> MAALGHTLP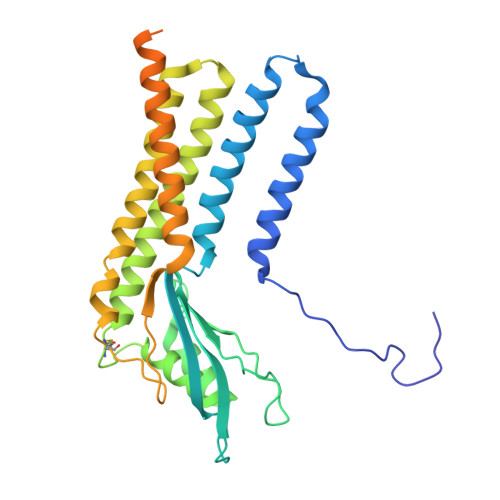FYTGTKPTFPMDTTLAVIITIFLTALVTFIIILPGIRGKTRLFWLLRVVTSLFIGAVILAVNFSSEWSVGHVNANTTYKAFSPKWVSVDVGLQIGLGGVNITLTGTPVQQLNETINYNEAFAWRLGRSYAEEYAKALEKGLPDPVLYLAEKFTPRSPCGLYNQYRLAGHYASAMLWVAFLCWLLANVMLSMPVLVYGGHMLLATGLFQLLALFFFSMTTSLISPCPLRLGTAVLHTHHGPAFWITLATGLLCILLGLVMAVAHRMQPHRLKAFFNQSSEDPVLEWGSEEGGLLSPHYRSIAESPETQDIPMSVASSETCFKEEHPKESDCSL> MSEIGTGFPFDPHYVEVLGERMHYVDVGPRDGTPVLFLHGNPTSSYLWRNIIPHVAPSHRCIAPDLIGMGKSDKPDLDYFFDDHVRYLDAFIEALGLEEVVLVIHDWGSALGFHWAKRNPERVKGIACMEFIRPFPTWDEWPEFARETFQAFRTADVGRELIIDQNAFIEGALPKYVVRPLTEVEMDHYREPFL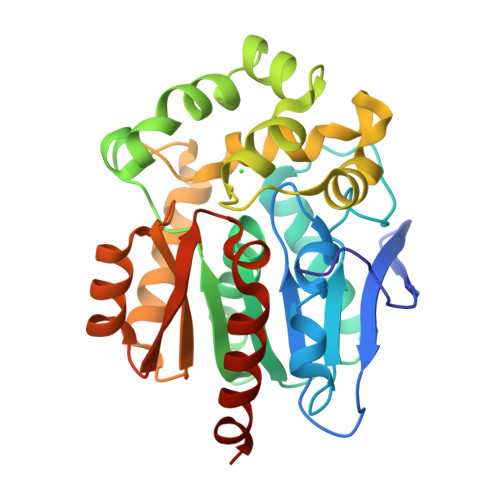KPVDREPLWRFPNELPIAGEPANIVALVEAYMNWLHQSPVPKLLFWGTPGFIIPPAEAARLAESLPNCKTVDIGPGLHFLQEDNPDLIGSEIARWLPALHHHHHH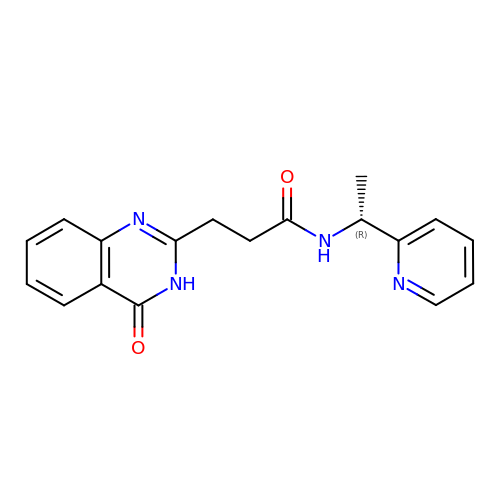3-(4-oxo-3,4-dihydroquinazolin-2-yl)-N-[(1R)-1-(pyridin-2-yl)ethyl]propanamide | C18 H18 N4 O2 | HWTVYWVFOWWESR-GFCCVEGCSA-N>[2x]GAITKAVFDNEQGQAQRLQTSSSVEHGQMLFKDANLKTPSDVLNAFAKLDSKMVKSHAAELSQLAERAMTEVML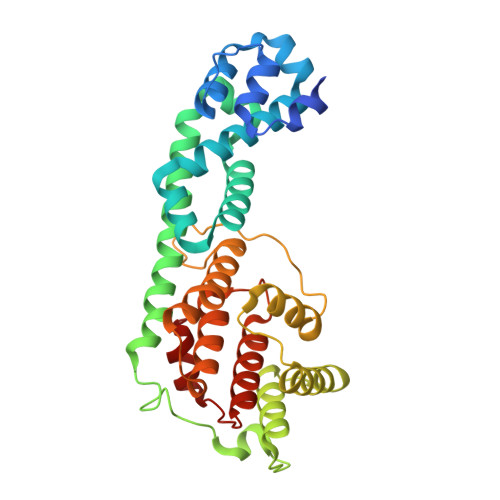ETDSGKNLKALIGDDAVKSLAVRVVKDYGGGVAAAQKNPEVRINQMQAVFDMEVMHLKAAQRHIEGLASTDLNQGVYAEGLPEDAFNKAGVTNNVERAAAWIINASNSKGNDAENITSLLKEYATNGKDLLNMDNLKELHARLVPNVERDYRGPNISGGTLPSSIGGEGMLKQHIEGFLKENPVADKDLGKHLFAGVIGYHGFTDGNGRMGRMLYAIAELRNDSFNPLAMNAENSLHGIK> T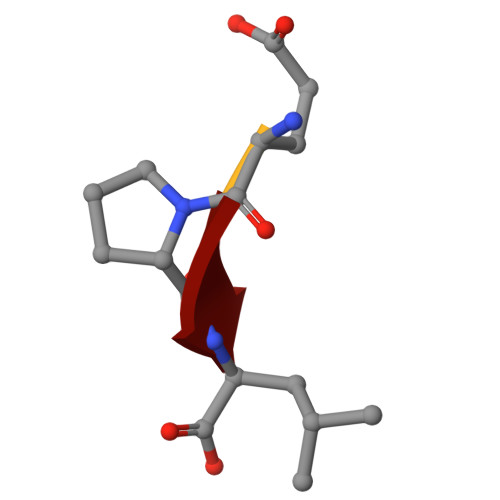EPL6~{H}-benzo[c][1,2]benzothiazine 5,5-dioxide | C12 H9 N 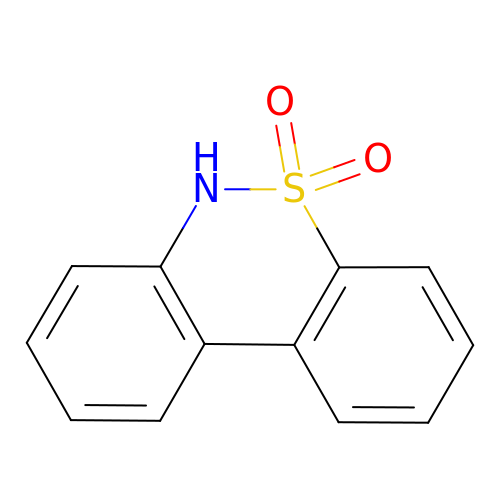O2 S | HXNJMXAYTVQMJT-UHFFFAOYSA-N>[3x]MGSSHHHHHHSSGRENLYFQGSATASELLLTAALERIEDTAQAMLSTVIDEERNPFLEGAPSYLPGKRPTDVTTFGQVPALRDMLAESRDLEFLQRVSDMAGPSPRIEDPSEEGLARHY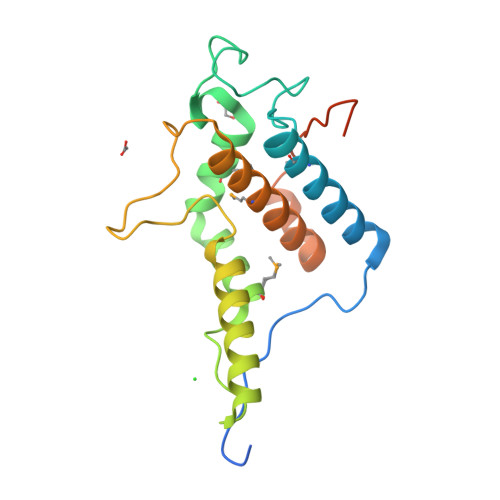TNVSNWKAQKSAHLGIVDHLGQFVYHEGSPLDVATLAKAVQMWKTRELIVHAHPQDRARFPELAVHIPEQVSDDSDSEQQTSPEPSGHQ> ANPLYQKHIISINDLSRDDLNLVLATAAKLKANPQPELLKHKVIASCFFEAST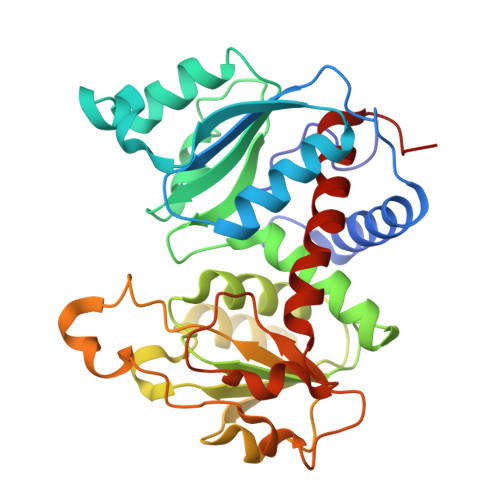RTRLSFETSMHRLGASVVGFSDSANTSLGKKGETLADTISVISTYVDAIVMRHPQEGAARLATEFSGNVPVLNAGDGSNQHPTQTLLDLFTIQQTQGRLDNLHVAMVGDLKYGRTVHSLTQALAKFDGNRFYFIAPDALAMPEYILDMLDEKGIAWSLHSSIEEVMAEVDILYMTRVQKERLDPSEYANVKAQFVLRASDLHNAKANMKVLHPLPRVDEIATDVDKTPHAWYFQQAGNGIFARQALLALVLNRDLVL> MNRPSGRAADQLRPIRITRHYTKHAEGSVLVEFGD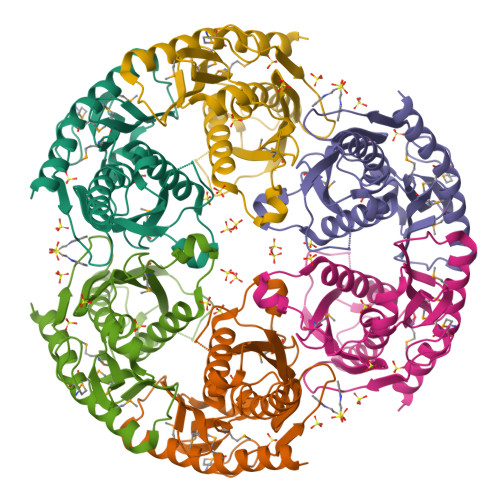TKVICTVSAESGVPRFLKGQGQGWLTAEYGMLPRSTGERNQREASRGKQGGRTLEIQRLIGRSLRAALDLSKLGENTLYIDCDVIQADGGTRTASITGATVALIDALAVLKKRGALKGNPLKQMVAAVSVGIYQGVPVLDLDYLEDSAAETDLNVVMTDAGGFIEVQGTAEGAPFRPAELNAMLELAQQGMQELFELQRAALAE4-(dimethylamino)benzohydrazide | C9 H13 N3 O | 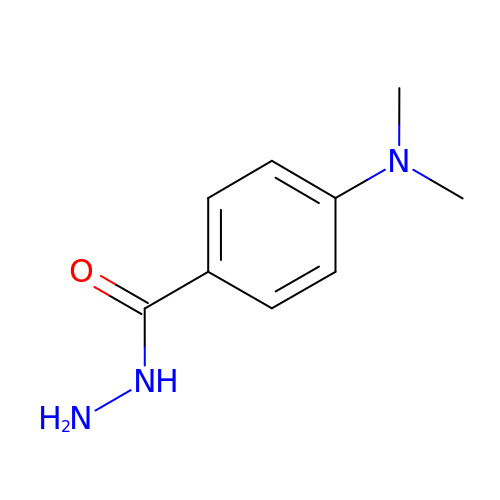HITIGLAGJBMISF-UHFFFAOYSA-N>MGVTKTTTQQGTGPSPQVGQTVVIEYTGFLKDTSKPDNKGAQFDSSVGRGDFETAIGVQRVIKGWDEGVVSMKVGEKATLDITADYGYGARGFPGAIPPNSDLIFDV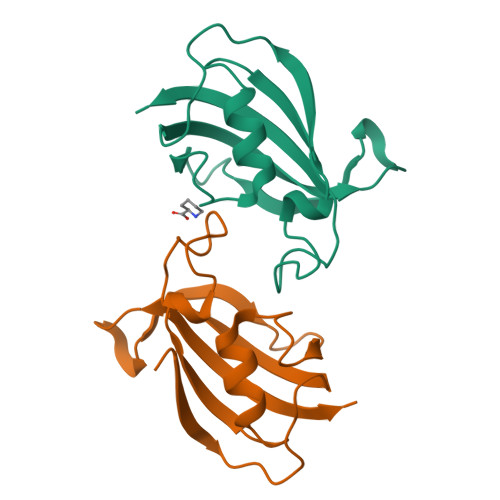YLKGIK[2x]(1S,5R)-2-(bromomethyl)-6,6-dimethylbicyclo[3.1.1]hept-2-ene | C10 H15 Br 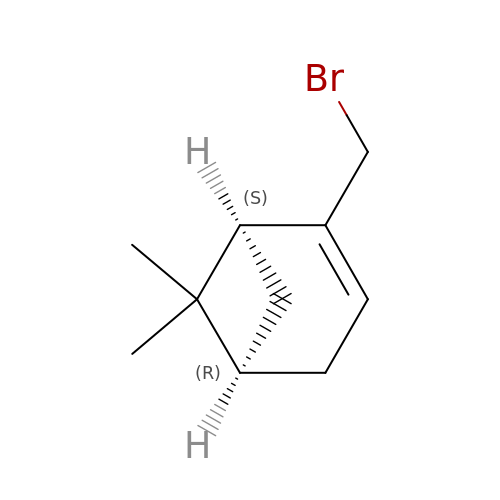| SNAIDRDMHGKCAX-RKDXNWHRSA-N>MATPVTIYGPPLSTAVSRVLATLIEKDVPFHLIPIDLSKGEQKKPEYLKIQPFGQVPAFKDESITLFESRAICRYICDKYADKGNKSLYGTDILSKANIDQWVETDGQTFGPPSGDLVHDLLFSSVPVDEALIKKNVDKLAKVLDIYEQKLGQTRFLAGDEFSFADLSHLPNGDYLVNSTDKGYLFTSRKNVNRWWTEISNRESWKKVLEMRKNA[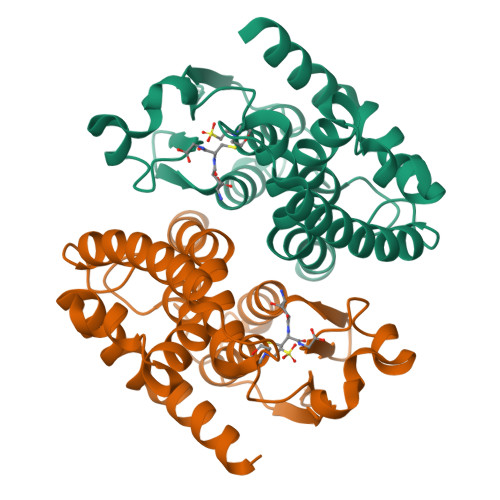2x]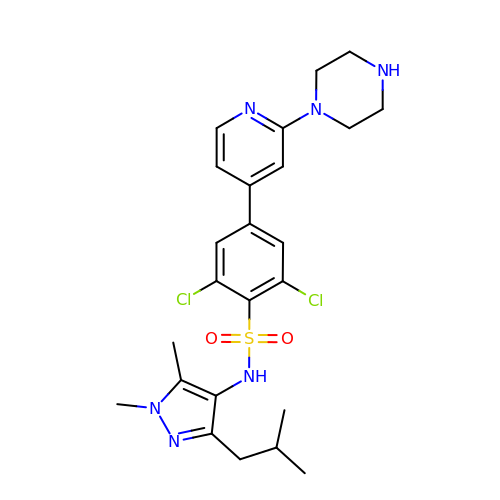2,6-DICHLORO-4-(2-PIPERAZIN-1-YLPYRIDIN-4-YL)-N-(1,5-DIMETHYL,3-ISOBUTYL-1H-PYRAZOL-4-YL)BENZENESULFONAMIDE | C24 H30 Cl2 N6 O2 S | WKTSLVQYGBHNRV-UHFFFAOYSA-N>[2x]MAHHHHHHMQLLDTLEQGLKEIDARGLRRRRRTVDSPCSAHMTVDGRNMIGFASNDYLGLAAHPLLVAAITEGARRYGAGSGGSHLLGGHSRAHAQLEDDLAEFAGGFVDNPRALYFSTGYMANLATLTALAGRGTTLFSDSLNHASLIDGARLSRADIQIYPHADAEALGAMLEASDAAVKLIVSDTVF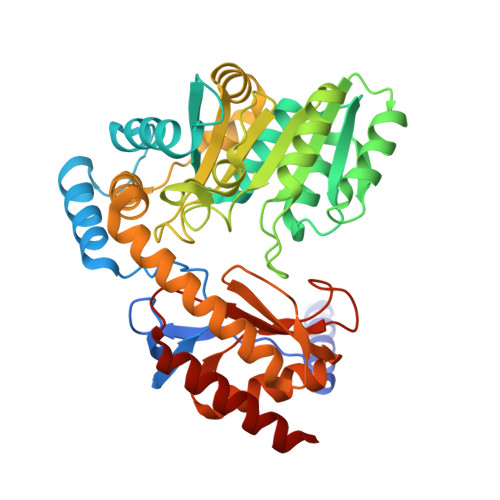SMDGDIAPLARLLELAEHHGAWLVVDDAHGFGVLGPQGRGAVAEAALRSPHLIVVGTLGKAAGVSGAFVVAHETVIEWLVQRARPYIFTTASVPSAAHAVSASLRIIGGDEGEHRRAHLRSLIALTRDMLKSTPWLPVDSHTAVQPLIIGSNEATLDVAASLDRANLWVPAIRPPTVPEGTSRLRISLSAAHSHNDLEQLEHALMKTAEARA> GSHMRKTLVLLGAHGVGRRHIKNTLITKHPDRFAYPIPHTTRPPKKDEENGKNYYFVSHDQ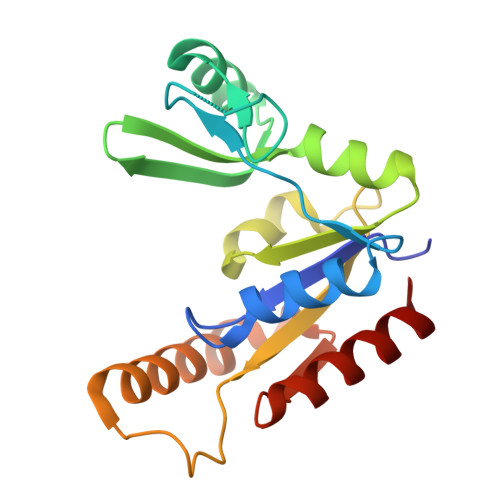MMQDISNNEYLEYGSHEDAMYGTKLETIRKIHEQGLIAILDVEPQALKVLRTAEFAPFVVFIAAPTITPGLNEDESLQRLQKESDILQRTYAHYFDLTIINNEIDETIRHLEEAVELVC>MQARKLAVDGAIEFTPRVFADDRGLLILPYQEEAFVEAHGGPLFRVAQTIHSMSK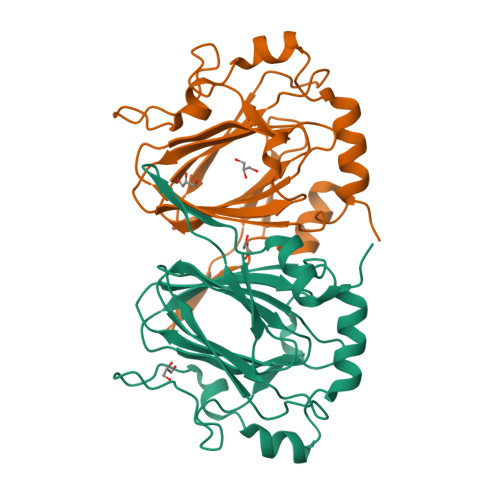RGVVRGIHYTVTPPGTAKYVYCARGKAMDIVIDIRVGSPTFGQWDSVLMDQQDPRAVYLPVGVGHAFVALEDDTVMSYMLSRSYVTQDELALSALDPALGLPIDIGVEPIVSDRDRVAITLAEAQRQGLLPDYTTSQEIERRLTAVPVST[2x]>[2x]MAETPNSDMSGATGGRSKRPKSNQDWWPSKLNLEILDQNARDVGPVEDDFDYAEEFQKLDLEAVKSDLEELMTSSQDWWPADYGHYGPLFIRMAWHSAGTYRTADGRGGAAGGRQRF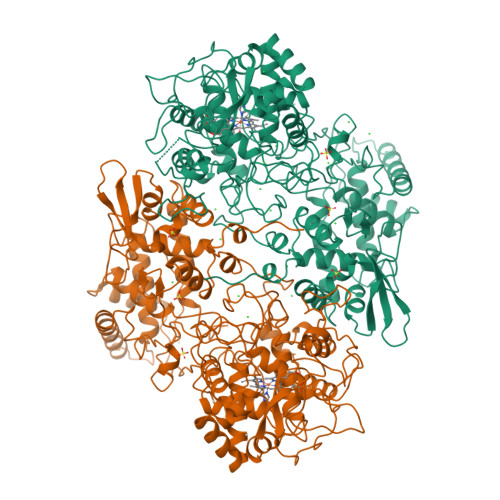APINSWPDNANLDKARRLLLPIKQKYGQKISWADLMILAGNVAIESMGFKTFGYAGGREDAFEEDKAVNWGPEDEFETQERFDEPGEIQEGLGASVMGLIYVNPEGPDGNPDPEASAKNIRQTFDRMAMNDKETAALIAGGHTFGKVHGADDPEENLGPEPEAAPIEQQGLGWQNKNGNSKGGEMITSGIEGPWTQSPTEWDMGYINNLLDYEWEPEKGPGGAWQWAPKSEELKNSVPDAHDPDEKQTPMMLTTDIALKRDPDYREVMETFQENPMEFGMNFAKAWYKLTHRDMGPPERFLGPEVPDEEMIWQDPLPDADYDLIGDEEIAELKEEILDSDLSVSQLVKTAWASASTYRDSDKRGGANGARLRLEPQKNWEVNEPEQLETVLGTLENIQTEFNDSRSDGTQVSLADLIVLGGNAAVEQAAANAGYDVEIPFEPGRVDAGPEHTDAPSFDALKPKVDGVRNYIQDDITRPAEEVLVDNADLLNLTASELTALIGGMRSIGANYQDTDLGVFTDEPETLTNDFFVNLLDMGTEWEPAADSEHRYKGLDRDTGEVKWEATRIDLIFGSNDRLRAISEVYGSADAEKKLVHDFVDTWSKVMKLDRFDLE>[4x]P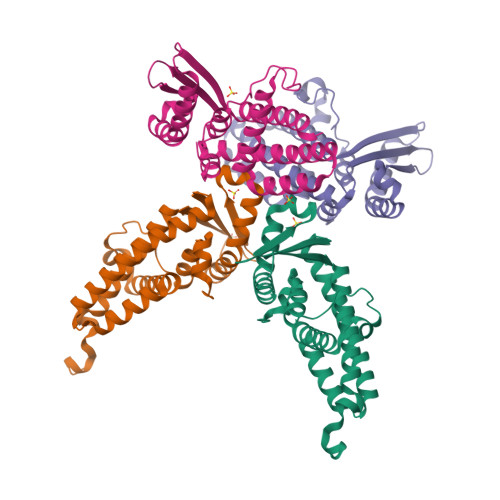DFTGARERFLAGDVTIVLLIAESHDAPYRLANPEDPEADLSDEQLERALAAYLTLVETLFPELYAEMKAALAAAKTPEEKIAVFREYNARFLAEFDALIDQAFARLKADSLTLKIHLSQGKGSYEIIFPPEVQADPERAAAIEALWKPTLDQLLAVLQEKHKGKPATTVTYEISAETLRAAVAALARAAEAALRRKVGSLESSGLEVLFQ>[2x]GHMKASSRRTISQNKRRYRKDGFDLDLTYVTDHVIAMSFPSSGRQSLFRNPIGEVSRFFKTKHP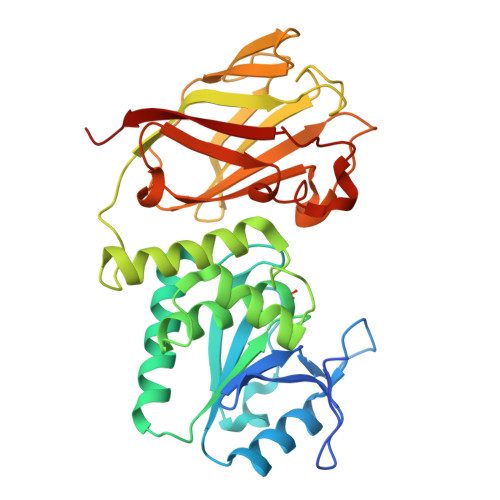DKFRIYNLCSERGYDETKFDNHVYRVMIDDHNVPTLVDLLKFIDDAKVWMTSDPDHVIAIHSKGGKGRTGTLVSSWLLEDGKFDTAKEALEYFGSRRTDVFQGVETASQIRYVGYFEKIKKNYGGQLPPMKKLKVTGVTITAIQGVGRGNGSDLSMQIVSERQEVLLCKFAEGYNCALQYDATDDCVTCEVKNCPVLAGDIKVRFMSTSKSLPRGYDNCPFYFWFNTSLVEGDHVTLKREEIDNPHKKKTWKIYRDNFTVKLTFSDAEDI>[2x]MELKSTRHTKYLCNYHFVWIPKHRRNTLVNEIAEYTKEVLKSIAEELGCEIIALEVMPDHIHLFVNCPPRYAPSYLANYFKGKSA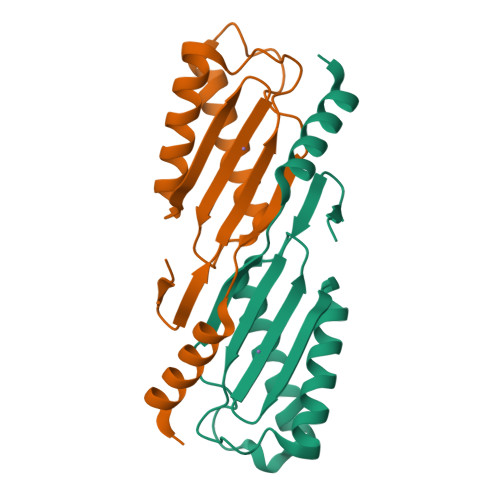RLILKKFPQLNKGKLWTRSYFVATAGNVSSEVIKKYIEEQWRKEGEEE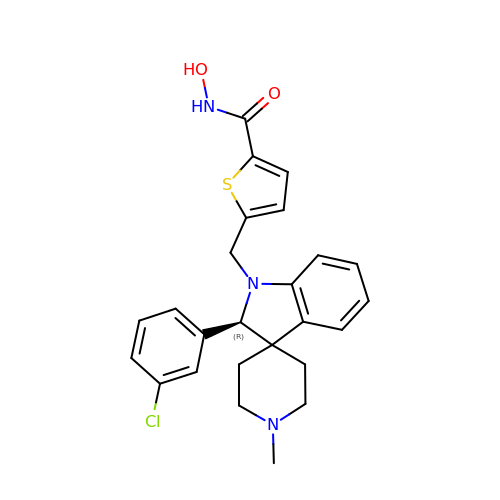5-[[(2R)-2-(3-chlorophenyl)-1'-methyl-spiro[2H-indole-3,4'-piperidine]-1-yl]methyl]-N-oxidanyl-thiophene-2-carboxamide | C25 H26 Cl N3 O2 S | JRHJYZJKMQDKEM-HSZRJFAPSA-N>[2x]MATQGVFTLPANTRFGVTAFANSSGTQTV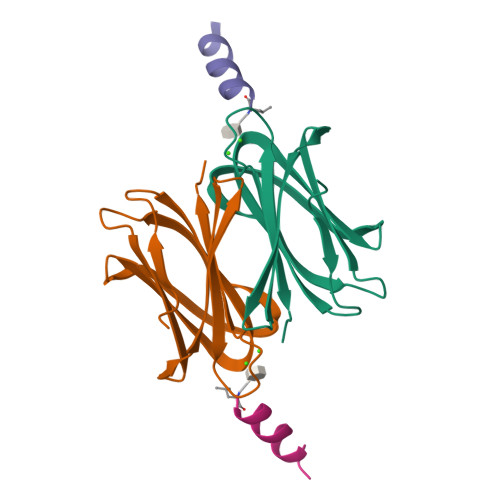NVLVNNETAATFSGQSTNNAVIGTQVLNSGSSGKVQVQVSVNGRPSDLVSAQVILTNELNFALVGSEDGTDNDYNDAVVVINWPLG;>LYKHFLKLFWLALX[2x]> AMRQCAIYGKGGIGKSTTTQNLVAALAEMGKKVMIVGCDPKADSTRLILHSKAQNTIMEMAAEAGTVEDLELEDVLKAGYGGVKCVESGGPEPGVGCAGRGVITAINFLEEEGAYEDDLDFVFYDVLGDVVCGGFAMPIRENKAQEIYIVCSGEMMAMYAANNISKGIVKYANSGSVRLGGLICNSRNTDREDELIIALANKLGTQMIHFVPRDNVVQ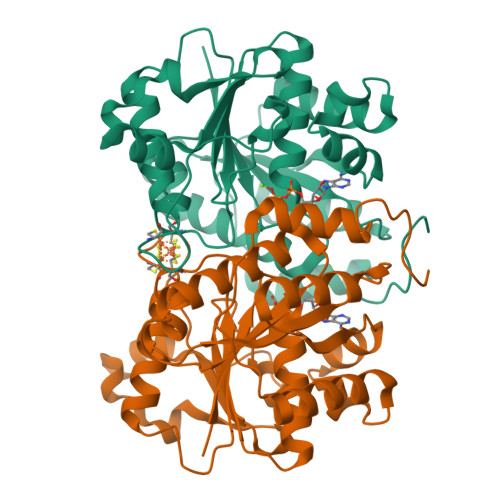RAEIRRMTVIEYDPKAKQADEYRALARKVVDNKLLVIPNPITMDELEELLMEFGIMEVEDESIVGKTAEEV>[6x]SKSVFVGELTWKEYEARVAAGDCVLMLPVGALEQHGHHMCMNVDVLLPTAVCQRVAERIGALVLPGLQYGYKSQQKSGGGNHFPGTTSLDGATLTGTVQDIIRELARHGVRRLVLMNGHYENSMFIVEGIDLALRELRYAGIHDFKVV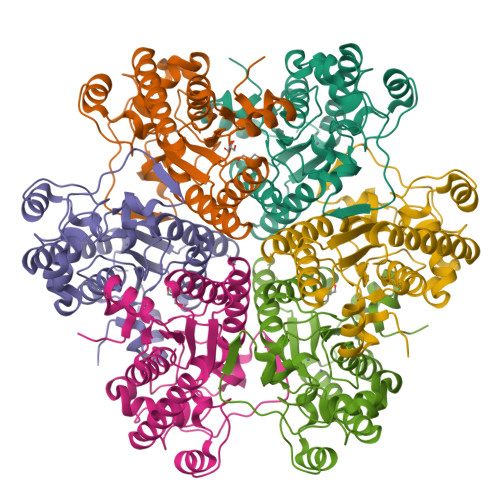VLSYWDFVKDPAVIQRLYPEGFLGWDIEHGGVFETSLMLALYPDLVDLERVVDHPPATFPPYDVFPVDPARTPAPGTLSSAKTASREKGELILEVCVQGIADAIGQEFPPT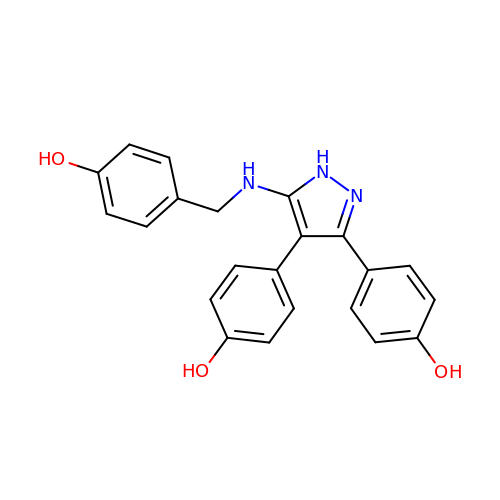4,4'-(5-{[(4-hydroxyphenyl)methyl]amino}-1H-pyrazole-3,4-diyl)diphenol | C22 H19 N3 O3 | YRRFETZFOOWFGO-UHFFFAOYSA-N> MTIKNYEVVIKTLGPIHIGSGQVMKKQDYIYDFYNSKVYMINGNKLVKFLKRKNLLYTYQNFLRYPPKNPRENGLKDYLDAQNVKQSEWEAFVSYSEKVNQGKKYGNTRPKPLNDLHLMVRDGQNKVYLPGSSIKGAIKTTLVSKYNNEKNKDIYSKIKVSDSKPIDESNLAIYQKIDINKSEKSMPLY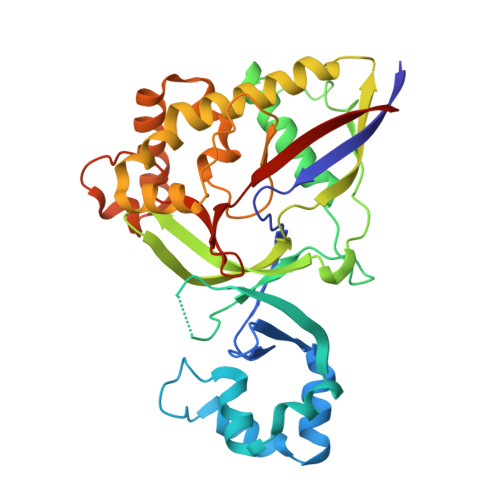RECIDVNTEIKFKLTIEDEIYSINEIEQSIQDFYKNYYDKWLVGFKETKGGRRFALEGGIPDVLNQNILFLGAGTGFVSKTTHYQLKNRKQAKQDSFEILTKKFRGTYGKMKEIPSNVPVALKGTTNQSRHTSYQQGMCKVSFQELNNEVL> LPQSVSRAAITAAYRRPETEAVSMLLEQARLPQPVAEQAHKLAYQLADKLRNQKNASGRAGMVQGLLQEFSLSSQEGVALMCLAEALLRIPDKATRDALIRDKISNGNWQSHIGRSPSLFVNAAT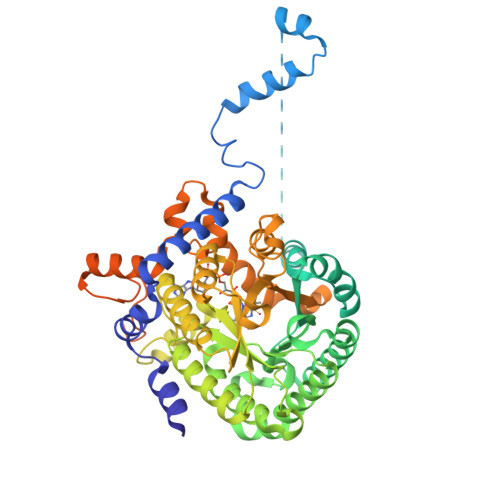WGLLFTGKLVSTHNEASLSRSLNRIIGKSGEPLIRKGVDMAMRLMGEQFVTGETIAEALANARKLEEKGFRYSYDMLGEAALTAADAQAYMVSYQQAIHAIGKASNGRGIYEGPGISIKLSALHPRYSRAQYDRVMEELYPRLKSLTLLARQYDIGINIDAEESDRLEISLDLLEKLCFEPELAGWNGIGFVIQAYQKRCPLVIDYLIDLATRSRRRLMIRLVKGAYWDSEIKRAQMDGLEGYPVYTRKVYTDVSYLACAKKLLAVPNLIYPQFATHNAHTLAAIYQLAGQNYYPGQYEFQCLHGMGEPLYEQVTGKVADGKLNRPCRIYAPVGTHETLLAYLVRRLLENGANTSFVNRIADTSLPLDELVADPVTAVEKLAQQEGQTGLPHPKIPLPRDLYGHGRDNSAGLDLANEHRLASLSSALLNSALQKWQALPMLEQPVAAGEMSPVINPAEPSSSVDKLAAALEHHHHHH METHYL 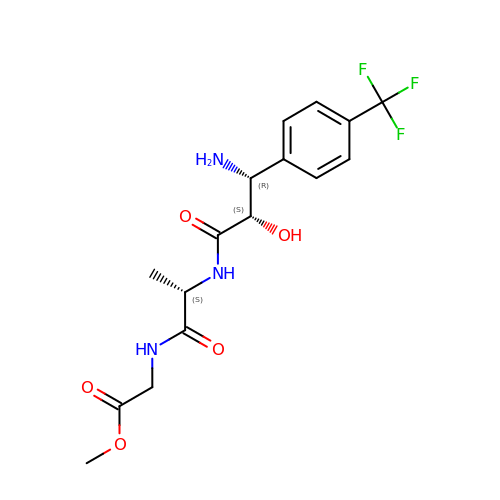N-{(2S,3R)-3-AMINO-2-HYDROXY-3-[4-(TRIFLUOROMETHYL)PHENYL]PROPANOYL}ALANYLGLYCINATE | C16 H20 F3 N3 O5 | KTNRONBAQGRLNO-CKLFPEKLSA-N> GMASAIIETAIPQSEMTASATSEEGQDPASSAIDGNINTMWHTKWNGSDALPQSLSVNLGKARKVSSIAITPRTSGNNGFITKYEIHAINNGVETLVAEGTWEENNLVKTVT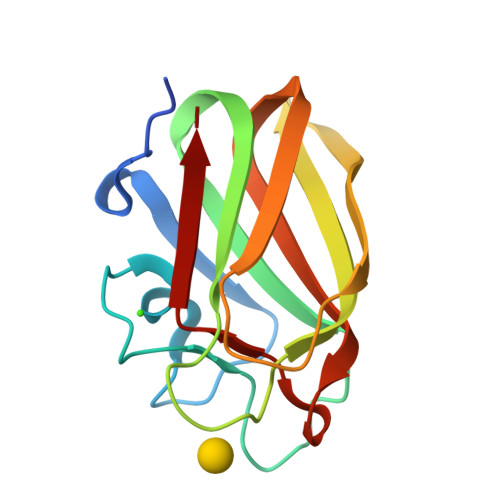FDSPIDAEEIKITAIQGVGGFASIAELNVYE>[2x]MASMTGGQQMGRDEAGITGTWYNQLGSTFIVTAGADGALTGTYESAVGN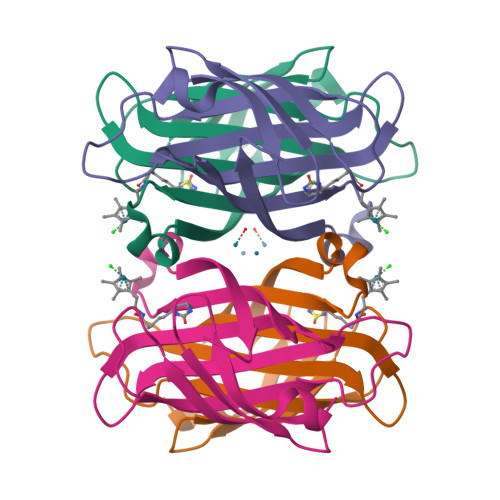AESRYVLTGRYDSAPATDGSGTALGWTVAWKNNYRNAHSATTWSGQYVGGAEARINTQWLLTSGTTEANAWHSTLVGHDTFTKVKPSAASIDAAKKAGVNNGNPLDAVQQ>[4x]MAMTGVLRPGHAQVRVLNLEEGIHFYRNVLGLVETGRDDQGRVYFKCWDERDHSCYIIREADTAGIDFFGFKVLDKATLEKLDADLQAYGLTTTRIPAGEMLETGERVRFELPS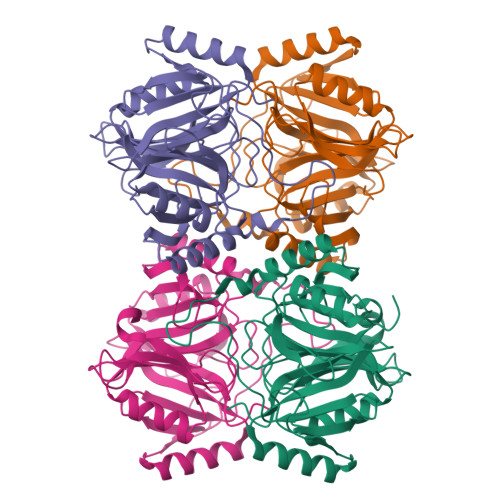GHLIELYAEKTCVGNGISEVNPAPWNAQREHGIAPIQLDHCLLYGPNIAEVQKIFTEVLGFYLVERVLSPDGDSDMGIWLSCSHKVHDIAFVEYPEKGKLHHCSFLLESWEQVLRAGDIMSMNEVNVDIGPTRHGVTRGCTIYAWDPSGNRFETFMGGYHPYPDYEPLSWTYDNFAQGLDYPQRKLHETFMTVVT>[4x]MHHHHHHAIGYVWNTLYGWVDTGTGSLAAANLTARMQPISHHLAHPDTKRRFHELVCASGQIEHLTPIAAVAATDADILRAHSAAHLENMKRVSNLPTGG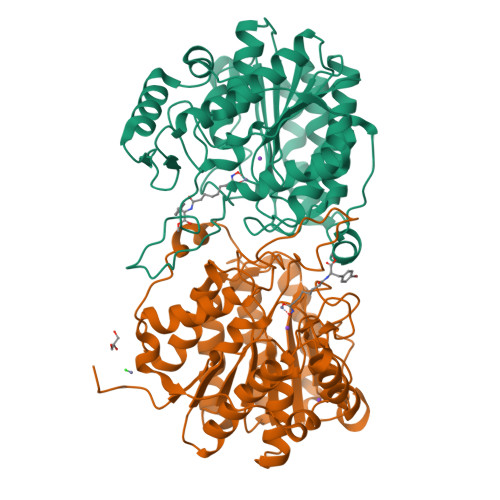DTGDGITMMGNGGLEIARLSAGGAVELTRRVATGELSAGYALVNPPGHHAPHNAAMGFCIFNNTSVAAGYARAVLGMERVAILDWDVHHGNGTQDIWWNDPSVLTISLHQHLCFPPDSGYSTERGAGNGHGYNINVPLPPGSGNAAYLHAMDQVVLPALRAYRPQLIIVGSGFDASMLDPLARMMVTADGFRQMARRTIDCAADICDGRIVFVQEGGYSPHYLPFCGLAVIEELTGVRSLPDPYHEFLAGMGGNTLLDAERAAIEEIVPLLADIR>[2x]MVKLKVEDLEMDKIAPLAPEVSLKMAWNIM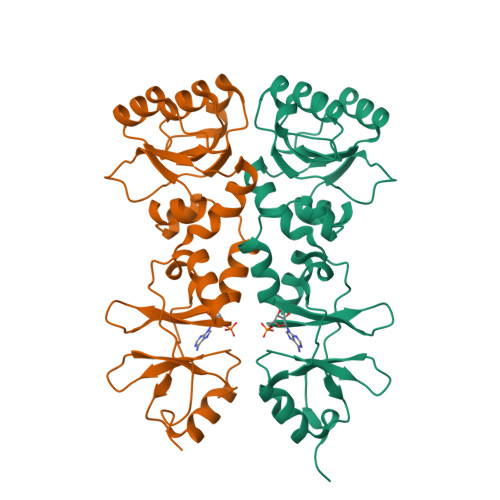RDKNLKSIPVADGNNHLLGMLSTSNITATYMDIWDSNILAKSATSLDNILDTLSAEAQNINEERKVFPGKVVVAAMQAESLKEFISEGDIAIAGDRAEIQAELIELKVSLLIVTGGHTPSKEIIELAKKNNITVITTPHDSFTASRLIVQSLPVDYVMTKDNLVAVSTDDLVEDVKVTMSETRYSNYPVIDENNKVVGSIARFHLISTHKKKLEHHHHHHHH>MRTV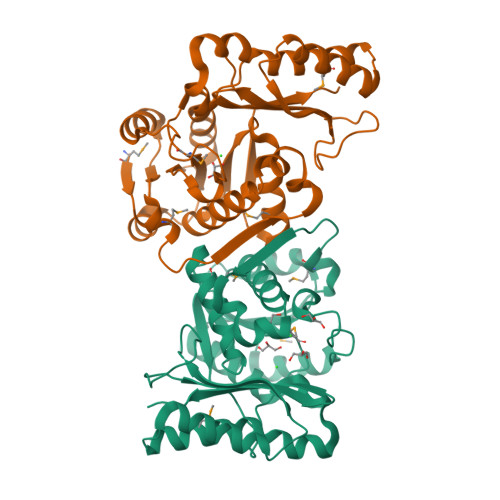STVAELRAALPREGVGFVPTMGYLHRGHLALVERARRENPFVVASVFVNPLQFGPGEDYHRYPRDLERDRALLQEAGVDLLFAPGVEEMYPEGFATRVQVEGPLTALWEGAVRPGHFQGVATVVARLFLLVQPQRAYFGEKDYQQLLVVRRMVRDLGFPVEVVGVPTVREEDGLALSSRNVYLSPETRKKAPVLYRALLAMREVAGQGGSVAEALRAGEEALRAVPEFRKDYLAIVHPETLLPLSDWVAGARGIVAGRFPEARLIDNLEVYP[2x]>GGEIRPTIGQQMETGDQRFGDLVFRQLAPNVWQHTSYLDMPGFGAVASNGLIVRDGGRVLVVDTAWTDDQTAQILNWIKQEINLPVALAVVTHAHQDKMGGMDALHAAGIATYANALSNQLAPQEGLVAAQHSLTFAANGWVEPATAPNFGPLKVFYPGPGHTSDNITVGIDGTDIAFGGCLIKDSKAKSLGNLDDADT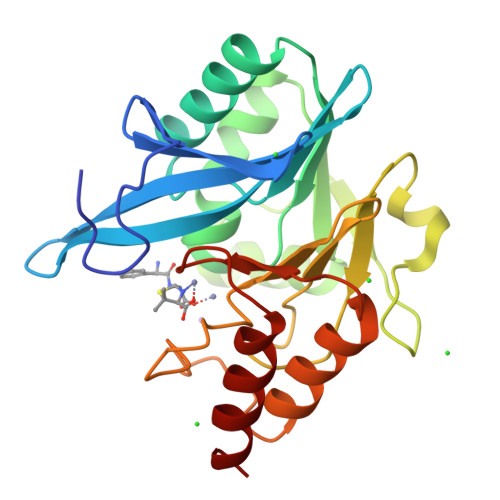EHYAASARAFGAAFPKASMIVMSHSAPDSRAAITHTARMADKLR[2x]>[6x]VVQGTVKPHASFNSREDAETLRKAMKGIGTDEKSITHILATRSNAQRQQIKTDYTTLFGKHLEDELKSELSGNYEAAALALLRKPDEFLAEQLHAAMKGLGTDKNALIDILCTQSNAQIHAIKAAFKLLYKEDLEKEIISETSGNFQRLLVSMLQGGRKEDEPVNAAHAAEDAAAIYQ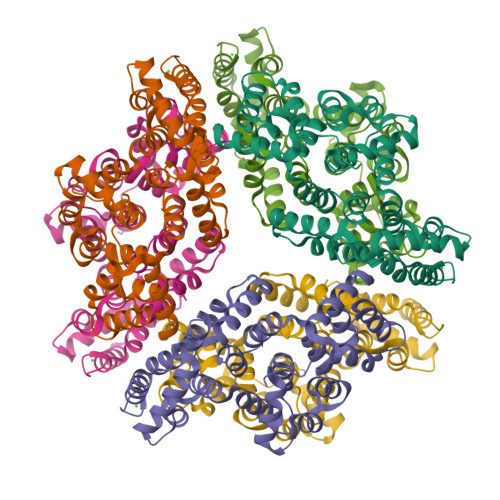AGEGQIGTDESRFNAVLATRSYPQLHQIFHEYSKISNKTILQAIENEFSGDIKNGLLAIVKSVENRFAYFAERLHHAMKGLGTSDKTLIRILVSRSEIDLANIKETFQAMYGKSLYEFIADDCSGDYKDLLLQITGH> MGHHHHHHMLHLLEQIRAYCETCWEWQEAHEPGMDQDKNPMPAPVEHQICPAVCVLMKLSFDEEHRHAMNELGGLQAIAELLQVDCEMYGLTNDHYSITLRRYAGMALTNLTFGDVANKATLCSMKGCMRALVAQLKSESEDLQQVIASVLRNLSWRADVNSKKTLREVGSVKALMECALEVKKESTLKSVLSALWNLSAHCTENKADICAVDGALAFLVGTLTYRSQTNTLAIIESGGGILRNVSSLIATNEDHRQILRENNCLQTLLQHLKSHSLTIVSNACGTLWNLSARNPKDQEALWDMGAVSMLKNLIHSKHKMIAMGSAAALRNLMANRPAKYKDANIMSPGSSLPS;> YQGGGEEMALP

Adenomatous polyposis coli (APC) is an important human tumor suppressor protein which plays critical roles in diverse cellular processes such as Wnt/β-catenin signaling, cell adhesion, cell migration, mitosis and chromosomal instability, and so on. The N-terminal armadillo repeat (ARM) domain of APC is the most conserved region among its vertebrate and invertebrate homologs, and mediates its association with a variety of binding partners including APC membrane recruitment 1 (Amer1, also named as WTX for ‘Wilms tumor gene on the X chromosome’), Asef, Sam68, and IQGAP1. By recruiting APC to the plasma membrane, Amer1 regulates the APC-dependent maintenance of intercellular junctions. In addition, together with APC and Axin, Amer1 promotes ubiquitination and degradation of β-catenin, thus negatively regulates the Wnt signal transduction pathway.

When the percentage of conservation for each Amer1 residue was carefully examined, another highly invariant sequence block between the A1 and A2 sites, residues 365–375, was found. Similar to the core A1 and A2 sequences, it also contains an acidic residue in the middle and several hydrophobic residues at its C-terminal part. To further understand the molecular basis of how APC recognizes Amer1, we determined the crystal structures of the APC–ARM/Amer1-A1, APC–ARM/Amer1-A2, and APC–ARM/Amer1-A4 complexes to 1.90 Å, 2.00 Å, and 1.70 Å resolutions, respectively. Despite possessing apparently different sequences, Amer1-A1, -A2, and -A4 adopt remarkably similar conformations when bound to APC–ARM, both in anti-parallel manners with respect to the armadillo repeats of APC. At all three interfaces between APC–ARM and Amer1-A1/A2/A4, four highly conserved asparagine residues, N507/N550/N594/N641 from the H3 helices of armadillo repeats 2/3/4/5 of APC–ARM function as rivets fastening Amer1-A1/A2/A4 onto its surface groove. In addition, two basic residues, APC-K516 and -R549, straddle the middle portion of Amer1-A1/A2/A4 peptides on both sides. They form salt bridges with a conserved acidic residue A1-D330/A2-D503/A4-E370 and make hydrogen bonds with the main chain carbonyl groups of A1-C328/A1-G329/A2-S501/A2-G502/A4-G368. Furthermore, a number of hydrophobic residues F458, M503, and F510 from APC cluster together and form hydrophobic contacts with non-polar residues such as I332/A333 from Amer1-A1, L505/T506 from Amer1-A2, and M372/A373 from Amer1-A4. Accordingly, point mutations of T326R/T326A, D330K/D330A, and I332D in Amer1-A1 eliminated its binding with APC–ARM; the S499A, D503K/D503A, and L505D mutations in Amer1-A2 undermined its complex formation with APC–ARM; and the E370K point mutation or deletion of residues 370–373 in Amer1-A4 eliminated its interaction with APC–ARM.(3R,4R)-4-{(3S,4S)-4-[6-chloro-2-({5-chloro-1-[(1R)-2,2-difluorocyclopropyl]-1H-pyrazol-4-yl}amino)quinazolin-7-yl]-3-fluoropiperidin-1-yl}oxolan-3-ol 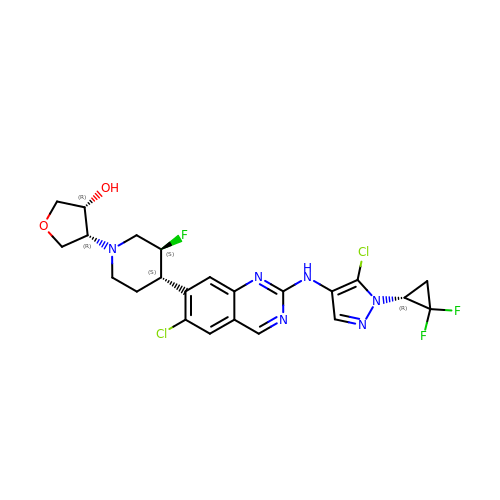| C23 H23 Cl2 F3 N6 O2 | JCYBYWFFRFKLHB-FYTJDIJESA-N>[2x]MRRIVVTGMGMINSLGLNKEDSFLAIAKGECGIKHIESFDASAFPVRIAGEITDFDPTEVMNPKDVKKAGRFIQLALKATREAMKDSGILDAHNRCPEELANRMGVSSGSGIGGLGNIEANSIFCFEKGPRKVNPFFITSALVNMIGGFTSIEFGIKGPNLSSVTACAAGTHAIIEAVKTILLNGADRMLVVGAESTICPVGIGGFASIKALSTRNDEPKKASRPFDKDRNG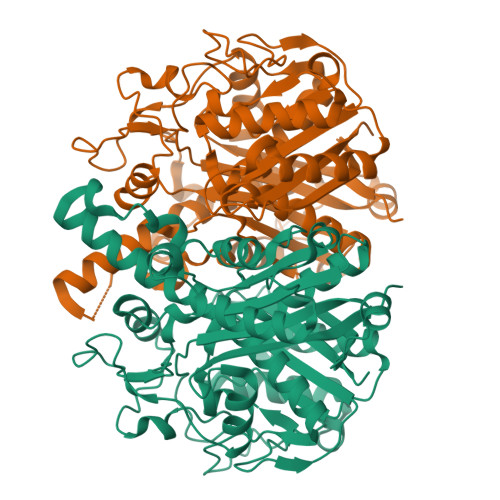FVMGEGAGALVLEEYESAKKRGAKIYAEFAGYGESGDANHITAPAPEGEGAFRAMKMALEMAKVEVGYVNAHGTSTHYNDLYESIALKNVFGSKEKVPPVSSTKGQIGHCLGAAGALEAVISIMAMNQGILPPTINQETPDPECDLDYIPNAAREKQVDAVMSNSFGFGGTNGVVIFKKA>[2x]GHHHHHHGENLYFQGASLTEIEHLVQSVCKSYRETCQLRLEDLLRQRSNIFSREEVTGYQRKSMWEMWERCAHH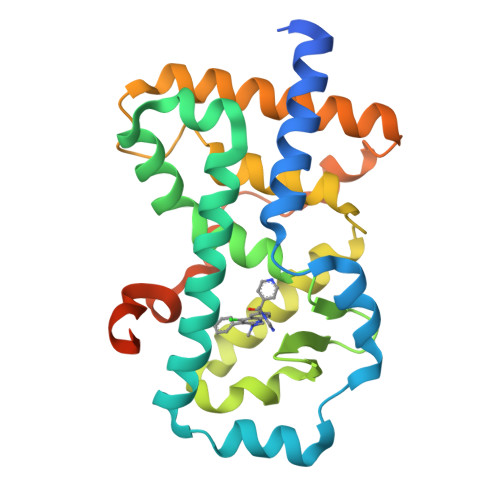LTEAIQYVVEFAKRLSGFMELCQNDQIVLLKAGAMEVVLVRMCRAYNADNRTVFFEGKYGGMELFRALGCSELISSIFDFSHSLSALHFSEDEIALYTALVLINAHRPGLQEKRKVEQLQYNLELAFHHHLCKTHRQSILAKLPPKGKLRSLCSQHVERLQIFQHLHPIVVQAAFPPLYKELFS>MSYYHHHHHHLESTSLYKKALAYTLPQLPYAYDALEPHIDARTMEIHHTKHHQTYVDNANKALEGTEFADLPVEQLIQQLDRVPADKKGALRNNAGGHANHSMFWQIMGQGQGQNGANQPSGELLDAINSAFGSFDAFKQKFEDAAKTRFGSGWAWLVVKDGKLDVVSTANQDNPLMGEAIAGVSGTPILGVDVWEHAYYLNYQNRRPDYLAAFWNV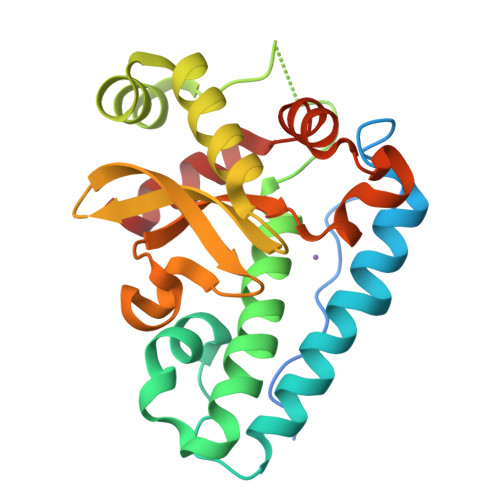VNWDEVSKRYAAAK[4x]>[2x]SLAANPWNWFGSSTKVSEQGVGELTASTPLQEQAIADALDGDYRLRSGMKTANG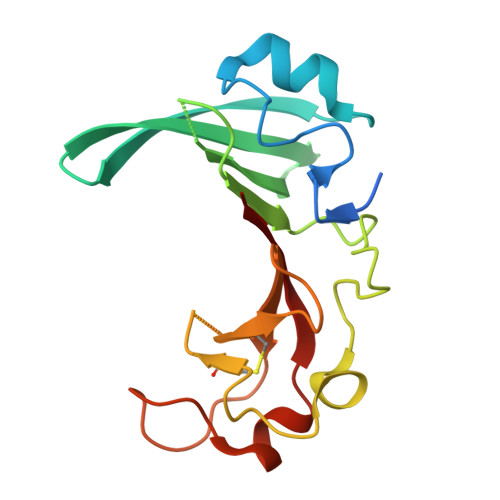NVVRFFEVMKGDNVAMVINGDQGTISRIDVLDSDIPADTGVKIGTPFSDLYSKAFGNCQKADGDDNRAVECKAEGSQHISYQFSGEWRGPEGLMPSDDTLKNWKVSKIIWRR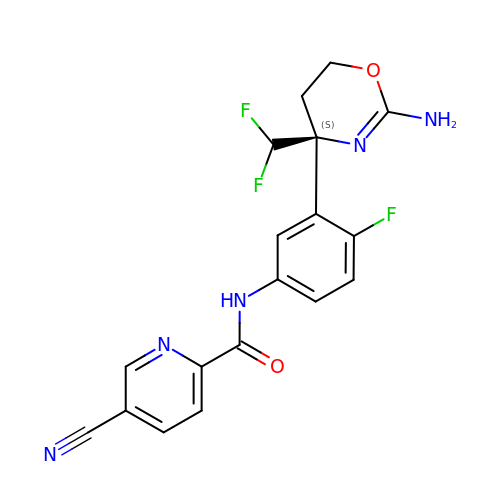N-{3-[(4S)-2-amino-4-(difluoromethyl)-5,6-dihydro-4H-1,3-oxazin-4-yl]-4-fluorophenyl}-5-cyanopyridine-2-carboxamide | C18 H14 F3 N5 O2 | ZQBDXEARYNLKKR-SFHVURJKSA-N In the gene cluster containing the lin1839 gene, the lin1840 gene encodes a putative glycoside hydrolase family (GH) 3 β-glucosidase (BGL) (GenBank accession number: CAC97071.1). The structure showed that Lin1840r forms a dimer of identical subunits each composed of three domains. The active center of Lin1840r is located at the interface of domains 1 and 2 as in the cases of known GH3 BGLs.

The crystal structure of apo wild-type (WT) Lin1840r was determined at 1.8 Å resolution. Lin1840r shows a similar overall structure to that of JMB19063. A loop (amino acids 568–598) in Lin1840r extends into the active site of the other subunit to form a part of the substrate pocket as in the case of the corresponding loop of JMB19063. Therefore, the formation of the dimer is predicted to be important for the catalysis. In domain 1, the N-terminal region of Lin1840r (amino acids 34–53) forms an α helix, whereas it forms a loop in JMB19063 (amino acids 29–48). In domain 2, the helix and loop (amino acids 435–455) extending to the active site in JMB19063 are missing in Lin1840r. In domain 3, clear electron density was observed. The metal ion obviously undergoes six-coordination with the side chain of Asp648, the backbone carbonyl of Thr650, and four water molecules. The two predicted catalytic residues, Asp270 and Glu473, occupy similar positions to the corresponding Asp residues (catalytic nucleophile) and Glu residues (catalytic acid/base), respectively, of the known enzymes. A distance between side chain carboxyl oxygen atoms of Asp270 and Glu473 is approximately 6.0 Å, suggesting that the enzyme follows retaining mechanism.

>[2x]MEQEKVQELVSQMTLDEKIAQCLQLSPFLFKGTNKNAELTGPLLQEMKLTDAHTENAGSVLGSSSALDMIGIQEAYLKTNRLGIPLVFMADVIHGYKTVFPIPLALGCSFDRETVRVMAEVSALEATADGHHVTFSPMLDLVRDPRWGRVMESTGEDPFLNSELGKAMVDGYQGDASKLNENLEQMAACVKHFAAYGAAEAGLEYNTVNMSTRELYQNYLPAYNAAIQAGAKLVMTAFNVVDGIPATMNKWLNRDVLRGEMEFDGVLISDWGAVAEVINHGTARNPKEAAQFSMEAGVDLEMMTTCYIHELKGLIEEGKLSENLLDEAVLRMLNLKNDLGLFEDPYRGLKNNDRTKDILTDESRGKARAAGVESAVLLENKSRLLPLAKEAKIALVGPLATSPDILGGWNVYGEEKDGINVETGLREVFETVEVVSTEYTELSEEDKVAVKAAVQNMDVVVLALGEKNEWGGEAGSLATIRLPEAQYQLAKFVQTLGKPVVITLFNGRPLEVKELAESSDALLELWFPGTEAGRVTADLLSGASNPSGKLSMSFPQTTGQIPVYYNHLRTGRPQTPENKGERYVSHYLDIPNEPFYPFGYGKSYSEFELKTSSLPKELNLGESLHVEVTIKNISDIAGKEVIQVYLQDVTASISRPVKELKAFEKVALQAGEEKTVTFELTSEAFSFYNHQLEKVQEPGLHRVFVGTSSEDVDVFEVEVGGYVLEHHHHHH>[2x]MNLPTAQEVQGLMARYIELVDVGDIEAIVQMYADDATVENPF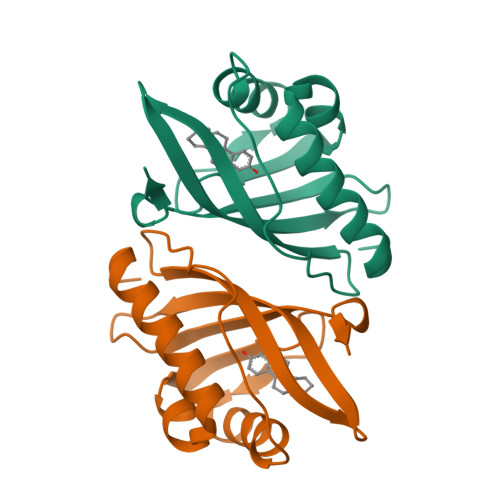GQPPIHGREQIAAFYRQGLGGGKVRACLTGPVRASHNGCGAMPFRVEMVWNGQPCALDVIDVMRFDEHGRIQTMQAYWSEVNLSVREPQ>[4x]MIQIYHADAFEIIKDFYQQNLKVDAIITDPPYNISVKNNFPT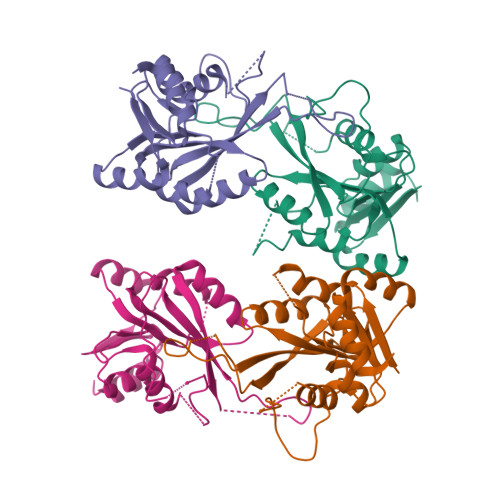LKSAKRQGIDFGEWDKNFKLLEWIARYAPLVNPNGCMVIFCSYRFISYIADFLEENGFVVKDFIQWVKNNPMPRNIHRRYVQDTEFALWAVKKKAKWVFNKPKNEKYLRPLILKSPVVSGLEKTKHPTQKSLALMEKIISIHTNPNDIVLDPFMGSGTTGLACKNLERNFIGIESEKEYFQTAKKRLNLFLEHHHHHH>SNAMAAIDLAREYISRVNGRDGSGAAALFAQDGEIIAPVGRVYRGWDAIAAFIEAAPPATTAQIAERTMGTHRVVLHGVVQTPRFAPAQIEWIFDVDGDRIRRLTINHLRD[4x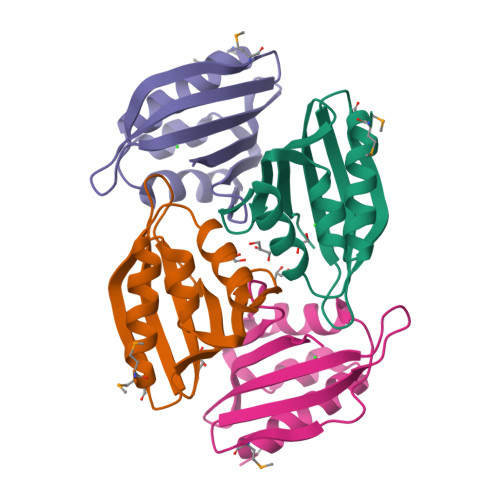]> GEIAALAVNAWKTTALKNAIAAAQKAGDAAGKIAGESKGVETIIGILEQYYSIYELKGTPLKSFFATTHYTDISNIATVIDTELNTSCGLNSLANQAICGLRTKLGL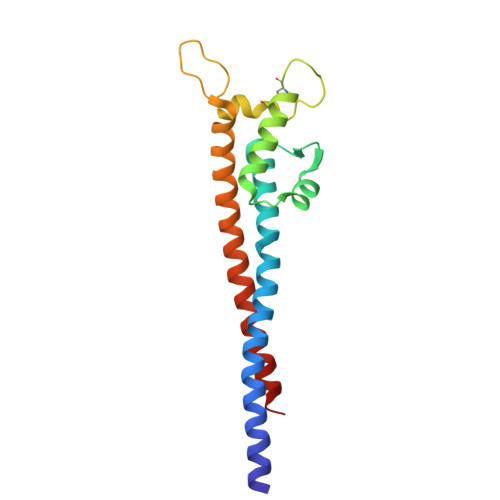VAKPGQVMVTQKEAITKMITNVVHKSEITAEAAKTEVAATKTAAAIKMNTEAIEAA> DMPVERILEAELAVEPKTETYVEANMGLNPSSPNDPVTNICQAADKQLFTLVEWAKRIPHFSELPLDDQVILLRAGWNELLIASFSHRSIAVKDGILLATGLHVHRNSAHSAGVGAIFDRVLTELVSKMRDMQMDKTELGCLRAIVLFNPDSKGLSNPAEVEALREKVYASLEAYCKHKYPEQPGRFAKLLLRLPALRSIGLKCLEHLFFFKLIGDTPIDTFLMEMLEAP;> HKILHRLLQD

RXRα interacts with different nuclear receptors to form heterodimers, thus executing different functions. The pleiotropic roles of RXRα have made this nuclear receptor an attractive target for drug discovery. Given that PPARγ partners with RXRα to form a “permissive” heterodimer, which can be activated by either RXRα or PPARγ modulator, it is possible that Rut increases the transcriptional activities of both RXRα:RXRα homodimer and PPARγ:RXRα heterodimer by activating RXRα or PPARγ. RXRα-LBD or PPARγ-LBD is reported to exhibit notably conformational changes upon agonist binding, subsequently recruiting its co-activator such as the steroid receptor coinducer-1 (SRC1).

Further target exploration research indicates that Rut functions as both a specific PTP1B inhibitor and an RXRα agonist that selectively activates PPARγ:RXRα heterodimer. Firstly, the binding affinity of Rut to the ligand-binding domain (LBD) of RXRα or PPARγ is determined using the surface plasmon resonance (SPR) technology based Biacore instrument. To study whether Rut is able to enhance the interaction between RXRα-LBD or PPARγ-LBD and the co-activator, the binding affinity of RXRα-LBD or PPARγ-LBD against SRC1613–773 containing the LXXLL motifs in the presence of different concentrations of Rut is measured. Subsequently, yeast two-hybrid assay is employed to further validate the effect of Rut on the co-activator recruitment. Considering that RXRα agonist 9-cis-retinoic acid could modulate GLUT4 promoter activity thereby increasing GLUT expression, we then test whether Rut is also able to increase GLUT4 promoter activity through targeting RXRα. Here, Rut is determined as a heterodimer-selective agonist. It activates PPARγ:RXRα but exhibits no effects on LXRα:RXRα or FXR:RXRα dimerization. Such a PPARγ:RXRα heterodimeric selectivity for Rut is expected to benefit its potential in drug development. Different from rosiglitazone and pioglitazone, the two members of thiazolidinedione (TZD) PPARγ agonists with anti-hyperglycemic activity, Rut could increase GLUT4 expression via enhancing RXRα-LBD/SRC1 interaction and PPARγ:RXRα heterodimer transcriptional activity through direct binding to RXRα.>[2x]A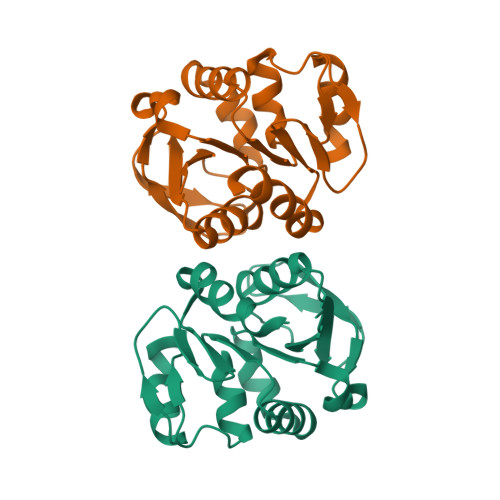SMKVLFLSADGFEDLELIYPLHRIKEEGHEVYVASFQRGKITGKHGYSVNVDLTFEEVDPDEFDALVLPGGKAPEIVRLNEKAVMITRRMFEDDKPVASICHGPQILISAKVLKGRRGTSTITIRDDVINAGAEWIDAEVVVDGNWVSSRHPGDLYAWMREFVKLLH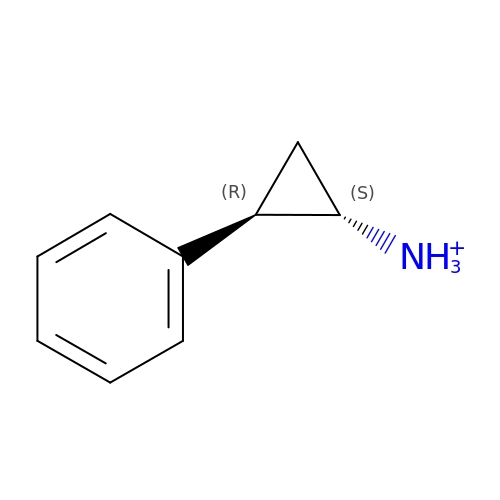TRANS-2-PHENYLCYCLOPROPYLAMINE | C9 H12 N | AELCINSCMGFISI-BDAKNGLRSA-O In this study, we identified aminoacyl-tRNA synthetase-mediated cap-dependent vertebrate-specific translation initiation machinery and investigated its structure, function, and molecular mechanism. TRS exhibits dual functionality to determine the vertebrate specificity of the machinery via its unique N-terminal extension that represents a gain-of-function component, and its ability to select target mRNAs. In the present study, we discovered that TRS regulates vertebrate-specific translation initiation. Thus, its association with either complex was somewhat diminished compared with the other components. These results suggest that TRS acts as an eIF4G-like scaffold and represents an eIF4F analog that acts independently of eIF4F.

The canonical motif of UNE-T is located in a position similar to that in the complexes of 4E-BP1–4EHP15, GIGYF1/2–4EHP15, 4E-BP1-eIF4E16, and eIF4G-eIF4E17. The residue corresponding to Lϕ in the consensus sequence is substituted by Mϕ in TRS. Residues Gly30−Asn48 in TRS were also not observed in the electron density map; hence these flexible regions were not included in the final model. Based on these results, we propose a schematic model for the TRS-mediated translation initiation machinery. The TRS ABD determines the selectivity of mRNAs by mimicking tRNA anticodon binding. PABP then integrates into the complex via interaction with the TRS ABD to form the efficient translation initiation machinery. Eventually, TRS links the complex to the ribosome via interaction with eIF3 to promote translation initiation. Herein, we identified a translation initiation machinery resulting from an evolutionary gain-of-function that is unique to vertebrates.

> KAVVPGPAEHPLQYNYTFWYSRRTPGRPTSSQSYEQNIKQIGTFASVEQFWRFYSHMVRPGDLTGHSDFHLFKEGIKPMWEDDANKNGGKWIIRLRKGLASRCWENLILAMLGEQFMVGEEICGAVVSVRFQEDIISIWNKTASDQATTARIRDTLRRVLNLPPNTIMEYKTHTDSIKMPGRLGPQRLLF;> GGKKKNKEGSGDGGRAELNPWPEYIYTRLEMYNILKAEHDSILAE>[4x]QVTF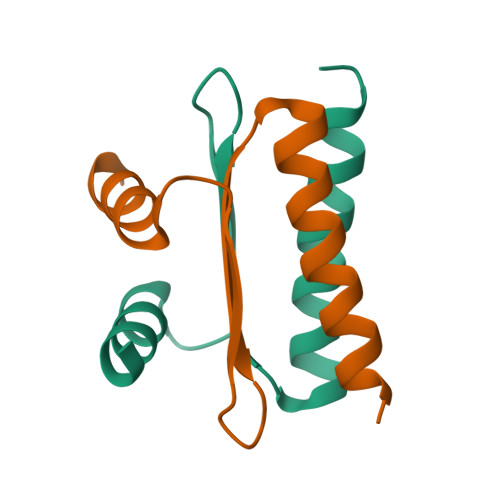AKRRNGLLKKAYELSVLCDAEVALIIFSNRGKLYEFCSSSSMLRTLERYQKCN> FPPQWICCDIRYLDVSILGKFAVVMADPPWDIHMELPYGTLTDDEMRRLNIPVLQDDGFLFLWVTGRAMELGRECLNLWGYERVDEIIWVKTNQLQRIIRTGRTGHWLNHGKEHCLVGVKGNPQGFNQGLDCDVIVAEVRSTSHKPDEIYGMIERLSPGTRKIELFGRPHNVQPNWITLGNQLDGIHLLDPDVVARFKQRYPDGIISKPKNL;> GTQSLNPHNDYCQHFVDTGHRPQNFIRDVGLADRFEEYPKLRELIRLKDELIAKSNTPPMYLQADIEAFDIRELTPKFDVILLEPPLEEYYRETGITANEKCWTWDDIMKLEIDEIAAPRSFIFLWCGSGEGLDLGRVCLRKWGYRRCEDICWIKTNKNNPGKTKTLDPKAVFQRTKEHCLMGIKGTVKRSTDGDFIHANVDIDLIITEEPEIGNIEKPVEIFHIIEHFCLGR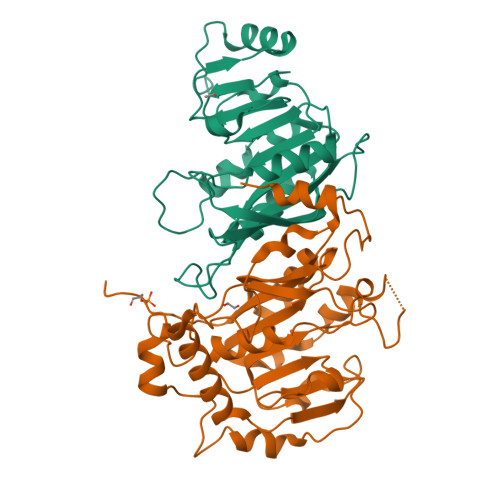RRLHLFGRDSTIRPGWLTVGPTLTNSNYNAETYASYFSAPNSYLTGCTEEIERLRPKSPPPKSKSDR> APDPLVKFSDVTVDLAARVIHRGEEEVHLTPIEFRLLAVLLNNAGKVLTQRQLLNQ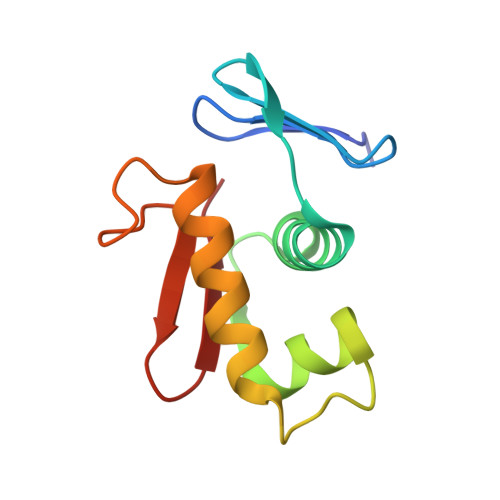VWGPNAVEHSHYLRIYMGHLRQKLEQDPARPRHFITETGIGYRFML>[2x]GHMASGPWKLTASKTHIMKSADVEKLADELHMPSLPEMMFGDNVLRIQHGSGFGIEFNATDALRCVNNYQGMLKVACAEEWQESRTEGEHSKEVIKPYDWTYTTDYKGTLLGESLKLKVVPTTDHIDTEKLKAREQIKFFEEVLLFE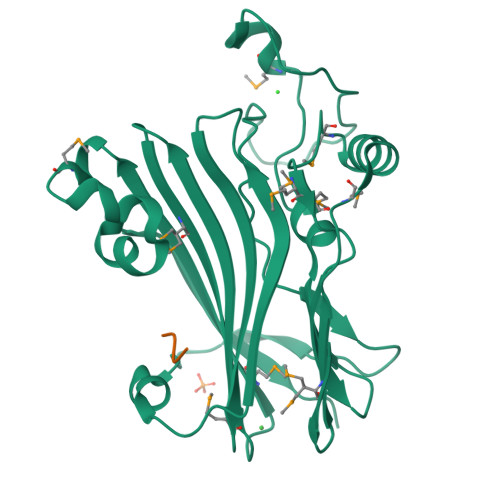DELHDHGVSSLSVKIRVMPSSFFLLLRFFLRIDGVLIRMNDTRLYHEADKTYMLREYTSRESKISSLMHVPPSLFTEPNEISQYLPIKEAVCEKLIFPE;>ENLYFQ[2x]> GPAGLVEGQNYTVLANPIPQQQAGKVEVLEFFGYFCPHCAHLEPVLSKHAKSFKDDMYLR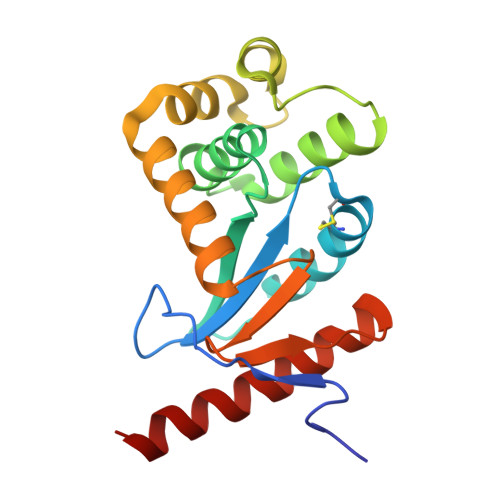TEHVVWQKEMLTLARLAAAVDMAAADSKDVANSHIFDAMVNQKIKLQNPEVLKKWLGEQTAFDGKKVLAAYESPESQARADKMQELTETFQIDGVPTVIVGGKYKVEFADWESGMNTIDLLADKVREEQKAAQ>[2x]GSSSGAGEGQGPKKQTRLGLEAKKEENLADWYSQVITKSEMIEYHDISGCYILRPWAYAIWEAIKDFFDAEIKKLGVENCYFPMFVSQSALEKEKTHVADFAPEVAWVTRSGKTELAEPIAIRPTSETVMYPAYAKWVQSHRDLPIKLNQWCNVVRWEFKHPQPFLRTREFLWQEGHSAFATMEEAAEEVLQILDLYAQVYEELLAIPVVKGRKTEKEKFAGGDYTTTIEAFISASGRAIQGGTSHHLGQNFSKMFEIVFEDPKIPGEKQFAYQNSWGLTTRTIGVMTMVHGDNMGLVLPPRVACVQVVIIPCGITNALSEEDKEALIAKCNDYRRRLLSVNIRVRADLRDNYSPGWKFNHWELKGVPIRLEVGPRDMKSCQFVAVRRDTGEKLTVAENEAETKLQAILEDIQVTLFTRASEDLKTHMVVANTMEDFQKILDSGKIVQIPFCGEIDCEDWIKKTTARDQDLEP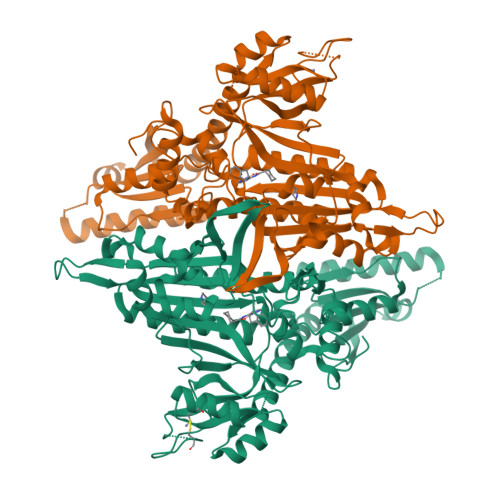GAPSMGAKSLCIPFKPLCELQPGAKCVCGKNPAKYYTLFGRSY6-Hydroxymethyl-7,8-dihydropterin pyrophosphokinase (HPPK, EC 2.7.6.3) catalyses pyrophosphoryl transfer from ATP (cofactor) to the substrate, 6-hydroxymethyl-7,8-dihydropterin (HMDP). HPPK is a small (158 residues, ∼18 kDa), generally monomeric protein and has been studied using various biophysical techniques, including x-ray crystallography and NMR spectroscopy. Three loop regions, loops L1–3, play an important role in substrate recognition and are critical for assembling the active centre. While loop L3 undergoes the largest and most dramatic conformational change during the catalytic cycle, all three loops help to seal the substrate and cofactor binding sites for the chemical transfer of a pyrophosphate from ATP to HMDP.

The x-ray crystal structure of SaHPPK in complex with the inhibitor, 8-mercaptoguanine was solved at high resolution. SaHPPK has a ferredoxin-like fold (αβα), with a central core of six β strands surrounded by four helices, typical of other monofunctional HPPK structures. The two monomers in the asymmetric unit are almost identical, with an RMSD of 0.34 Å over all 158 pairs of backbone Cα atoms. The catalytic loops L1, L2 and L3 (residues 12–14, 47–51, 82–94) have higher than average temperature factors, showing that they are likely mobile in solution, which parallels the observed broadening of residues in solution by NMR. The dimer interface encapsulates the active sites, leading to a buried surface area of 1595 Å, not including the inhibitor molecules. Like HMDP, the pyrimidine ring of 8-mercaptoguanine is stacked between the conserved aromatic residues, Phe54 and Phe123. A small cavity is found near the N7 position of 8-mercaptoguanine, in which a single water molecule resides, forming hydrogen bonds with the sidechain of Asp95 and the N7 of 8-mercaptoguanine. Notably, two of the interactions formed between HMDP and HPPK are absent in the case of 8-mercaptoguanine. Firstly, the imidazole ring of 8-mercaptoguanine is too far away to interact with Asp95, which forms a hydrogen bond with the hydroxymethyl group of HMDP.

>GSHMIQAYLGLGSNIGDRESQLNDAIKILNEYDGISVSNISPIYETAPVGYTEQPNFLNLCVEIQTTLTVLQLLECCLKTEECLHRIRKERWGPRTLDVDILLYGEEMIDLPKLSVPHPRMNERAFVLIPLNDIAANVVEPRSKLKVKDLVFVDDSVKRYK[2x]> MLPQRLHPSRLLALALFSLVLGLAGCQTKPPQTGLSAEQIAVLQEQGFELRDEGWEFGMSSKVLFGNNLDRLNPDSRNTLTKIARALLAVDIDKVRLEGHTDNYGDEGYNQKLSERRAESVAAVFREAGMPAANIEVRGLGMSKPVADNKTRAGRSENRRVAIIVPAE

The tripartite signalling system YfiBNR in P. aeruginosa modulates intracellular c-di-GMP levels in response to signals received in the periplasm and is a key regulator of the SCV phenotype. The effector protein YfiN (also known as TpbB or PA1120) is an integral inner membrane protein that functions as a diguanylate cyclase, consisting of a periplasmic PAS domain, a cytoplasmic HAMP domain and a catalytic GGDEF domain. The third component of the YfiBNR signalling system, YfiR, has a key role in the signal transduction process by bridging YfiN in the inner membrane and YfiB in the outer membrane. YfiB can release the repression of YfiN by sequestering YfiR at the outer membrane, which requires both membrane anchoring and peptidoglycan binding by YfiB for full activity.

Crystal structures of the periplasmic domain of YfiB were determined for two different constructs: from residues 27–168 to 1.58 Å resolution, and from residues 59–168 to 1.39 Å resolution. The YfiB(59–168) construct also excludes the region from residues 35–55 linked to increased membrane attachment. The longer YfiB construct crystallizes with two molecules in an asymmetric unit while the shorter construct crystallizes with only one molecule per asymmetric unit. Analytical ultracentrifugation data confirms that YfiB(27–168) predominantly forms a dimer in solution, while YfiB(59–168) is exclusively a monomer. The YfiB(59–168) structure lacks helix α1’ and strand β1’ and has a considerably shorter β1 strand than its larger counterpart, but otherwise retains the same core domain. The two structures can be superimposed with an r.m.s.d. of 1.3 Å for 105 aligned residues. The largest structural differences occur at the N-terminus, which dissociates from the β-sheet in YfiB(59–168), and in the β2-α2 loop, which packs against helix α3 in the shorter structure but is directed away from α3 in the longer structure. Strand β1’ and helix α1’ includes residues that are proposed to form a linker region that unfolds to facilitate membrane attachment and YfiR sequestration. This is consistent with our observations from structures of YfiB alone and in complex with YfiR that reveal structural rearrangements in this N-terminal linker region, including shortening of strand β1 in YfiB(59–168) and complete unfolding of β1 upon YfiR binding. The structure of P. aeruginosa YfiB(59–168) was determined by molecular replacement with Phaser using the YfiB(27–168) structure as a search model.> GAMGSGDTQLFNRAVSMVEKNKDIRSLLQCDDGITGKERLKAYGE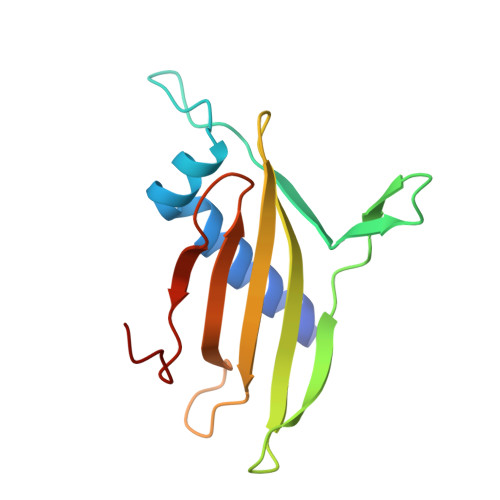LITNDKWTRNRPIVSTKKLDKEGRTHHYMRFHVESKKKIALVHLEAKESKQNYQPDFINMYVDVPGEKRYYLIKPKLHPVSN>PISPIETVPVKLKPGMDGPKVKQWPLTEEKIKALVEICTEMEKEGKISKIGPENPYNTPVFAIKKKDSTKWRKLVDFRELNKRTQDFWEVQLGIPHPAGLKKKKSVTVLDVGDAYFSVPLDEDFRKYTAFTIPSINNETPGIRYQYNVLPQGWKGSPAIFQSSMTKILEPFKKQNPDIVIYQYMDDLYVGSDLEIGQHRTKIEELRQHLLRWGLTTPDKKHQKEPPFLWMGYELHPDKWTVQPIVLPEKDSWTVNDIQKLVGKLNWASQIYPGIKVRQLCKLLRGTKALTEVIPLTEEAELELAENREILKEPVHGVYYDPSKDLIAEIQKQGQGQWTYQIYQEPFKNLKTGKYARMRGAHTNDVKQLTEAVQKITTESIVIWGKTPKFKLPIQKETWETWWTEYWQATWIPEWEFVNTPPLVKLWYQLEKEPIVGAETFYVDGAANRETKLGKAGYVTNKGRQKVVPLTNTTNQKTELQAIYLALQDSGLEVNIVTDSQYALGIIQAQPDKSESELVNQIIEQLIKKEKVYLAWVPAHKGIGGNEQVDKLVSAGIRKIL[4x];>PISPIETVPVKLKPGMDGPKVKQWPLTEEKIKALVEICTEMEKEGKISKIGPENPYNTPVFAIKKKDSTKWRKLVDFRELNKRTQDFWEVQLGIPHPAGLKKKKSVTVLDVGDAYFSVPLDEDFRKYTAFTIPSINNETPGIRYQYNVLPQGWKGSPAIFQSSMTKILEPFKKQNPDIVIYQYMDDLYVGSDLEIGQHRTKIEELRQHLLRWGLTTPDKKHQKEPPFLWMGYELHPDKWTVQPIVLPEKDSWTVNDIQKLVGKLNWASQIYPGIKVRQLCKLLRGTKALTEVIPLTEEAELELAENREILKEPVHGVYYDPSKDLIAE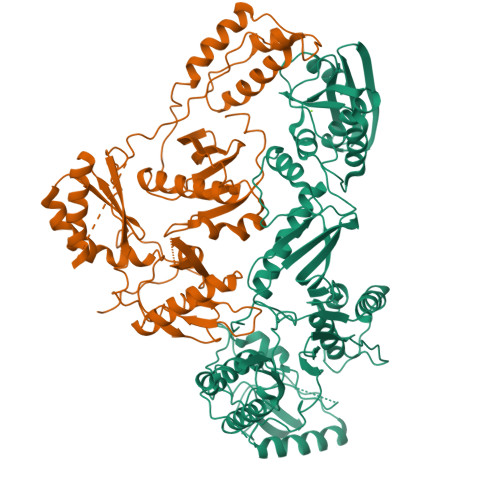IQKQGQGQWTYQIYQEPFKNLKTGKYARMRGAHTNDVKQLTEAVQKITTESIVIWGKTPKFKLPIQKETWETWWTEYWQATWIPEWEFVNTPPLVKLWYQLEKEPIVGAETF[4x]> MDPKISEMHPALRLVDPQIQLAVTRMENAVGRDQNNVGPKVYPIILRLGSPLSLNMARKTLNSLEDKAFQLTPIAVQMTKLATTEELPDEFVVVTVK;> MAASKPVEAAVVAAAVPSSGSGVGGGGTAGPGTGGLPRWQLALAVGAPLLLGAGAIYLWSRQQRRREARGRGDASGLKRNSERKTPEGRASPAPGSGHPEGPGAHLDMNSLDRAQAAKNKGNKYFKAGKYEQAIQCYTEAISLCPTEKNVDLSTFYQNRAAAFE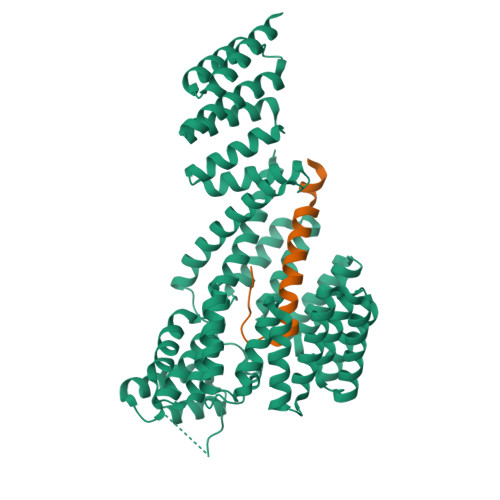QLQKWKEVAQDCTKAVELNPKYVKALFRRAKAHEKLDNKKECLEDVTAVCILEGFQNQQSMLLADKVLKLLGKEKAKEKYKNREPLMPSPQFIKSYFSSFTDDIISQPMLKGEKSDEDKDKEGEALEVKENSGYLKAKQYMEEENYDKIISECSKEIDAEGKYMAEALLLRATFYLLIGNANAAKPDLDKVISLKEANVKLRANALIKRGSMYMQQQQPLLSTQDFNMAADIDPQNADVYHHRGQLKILLDQVEEAVADFDECIRLRPESALAQAQKCFALYRQAYTGNNSSQIQAAMKGFEEVIKKFPRCAEGYALYAQALTDQQQFGKADEMYDKCIDLEPDNATTYVHKGLLQLQWKQDLDRGLELISKAIEIDNKCDFAYETMGTIEVQRGNMEKAIDMFNKAINLAKSEMEMAHLYSLCDAAHAQTEVAKKYGLKPPTL> MFEVPITLTNRKFAQRRKLKYQYINYISRRFDRISKKSTTTDSLPTPENSAAENNDEEEGQNSEAGTYRRSVLQQKKRRRERHWRSVVGEIYSTTESETDSQEEETEEGGEHDTGIDKEDSDEERKFWKKYEKPEKSFEIWRTVSSQNKQPINKQKMTYHNFKKIEKIPLRKMEIPLLHCTKENKLYFQSISRGLEPLKTSTSEVRNYRTRHIVTLTDLLHLNVSRHNWSLAYKIFATLIRIPGVQIKSLWGIGVEILDNLSNSSSGLDFLQWMCQIYSSKSRFVQNINYRSIVPPFQTGSRTHTAKFAITYLWSSLINCQKSMEPSSNIIDKPFDTENDLLQELIDKISEWVLTPPFMEDAEVWFIYASCHLLKADTLSRQFVNDNKNNDLIGLDRDIKINQVIKHIHYVRTFLKICLDKGGFAVPSRLIENQLKSFESRL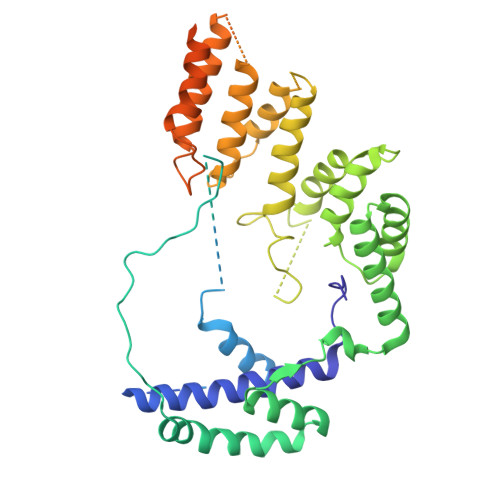YGEAQDIQERDVANVYDSIDNSSVENSFGDVYETNAEFLDTQLMDLSPEDNGLDEMHYSDEDSSE>GPGEKLELRLKSPVGAEPAVYPWPLPVYDKHHDAAHEIIETIRWVCEEIPDLKLAMENYVLIDYDTKSFESMQRLCDKYNRAIDSIHQLWKGTTQPMKLNTRPSTGLLRHILQQVYNHSVTDPEKLNNYEPFSPEVYGETSFDLVAQ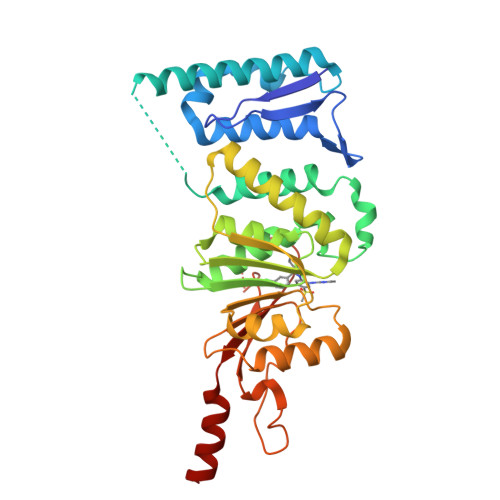MIDEIKMTDDDLFVDLGSGVGQVVLQVAAATNCKHHYGVEKADIPAKYAETMDREFRKWMKWYGKKHAEYTLERGDFLSEEWRERIANTSVIFVNNFAFGPEVDHQLKERFANMKEGGRIVSSKPFAPLNFRINSRNLSDIGTIMRVVELSPLKGSVSWTGKPVSYYLHTIDRTILENYFSSLKNPG[2x]>SYSTLANFPVQARNDNISPWTITGFADGESSFMLTVSKDSKRNTGWSVRPRFRIGLHNKDVTILKSIREYLGAGIITSDIDARIRFESLKELEVVINHFDKYPLITQKRADYLLFKKAFYLIKNKEHLTEEGLNQILTLKASLNLGLSEELKEAFPNTIPAERLLVTGQEIPDSNWVAGFTAGEGSFYIRIAKNSTLKTGYQVQSVFQITQDTRDIELMKNLISYLNCGNIRIRKYKGSEGIHDTCVDLVVTNLNDIKEKIIPFFNKNHIIGVKLQDYRDWCKVVTLIDNKEHLTSEGLEKIQKIKEGMNRGRS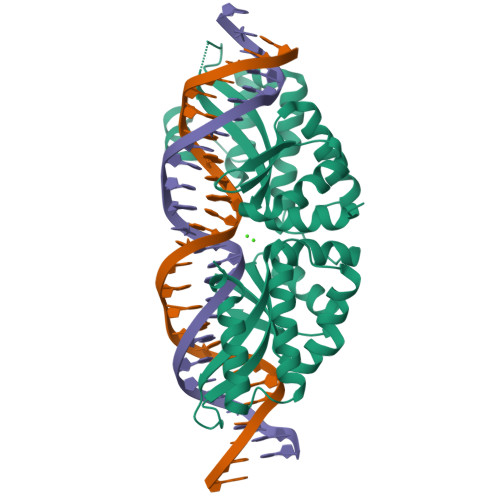L[4x]> NLDAAGFLQIWQHFDADDNGYIEGKELDDFFRHMLKKLQPKDKITDERVQQIKKSFMSAYDATFDGRLQIEELANMILPQEENFLLIFRREAPLDNSVEFMKIWRKYDADSSGYISAAEL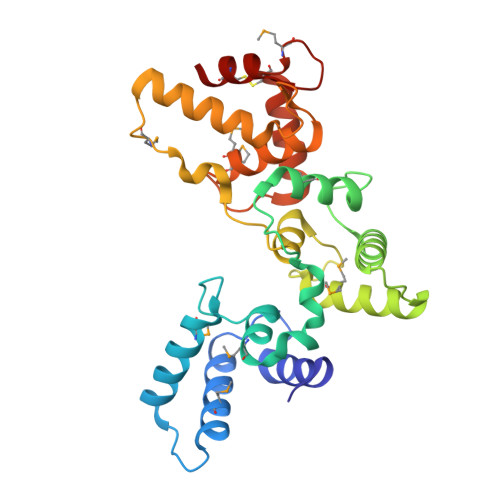KNFLKDLFLQHKKKIPPNKLDEYTDAMMKIFDKNKDGRLDLNDLARILALQENFLLQFKMDASSQVERKRDFEKIFAHYDVSRTGALEGPEVDGFVKDMMELVRPSISGGDLDKFRECLLTHCDMNKDGKIQKSELALCLG> MAKQLQARRLDGIDYNPWVEFVKLASEHDVVNLGQGFPDFPPPDFAVEAFQHAVSGDFMLNQYTKTFGYPPLTKILASFFGELLGQEIDPLRNVLVTVGGYGALFTAFQALVDEGDEVIIIEPFFDCYEPMTMMAGGRPVFVSLKPGPIQNGELGSSSNWQLDPMELAGKFTSRTKALVLNTPNNPLGKVFSREELELVASLCQQHDVVCITDEVYQWMVYDGHQHISIASLPGMWERTLTIGSAGKTFSATGWKVGWVLGPDHIMKHLRTVHQNSVFHCPTQSQAAVAESFEREQLLFRQPSSYFVQFPQAMQRCRDHMIRSLQSVGLKPLIPQGSYFLITDISDFKRKMPDLPGAVDEPYDRRFVKWMIKNKGLVAIPVSIFYSVPH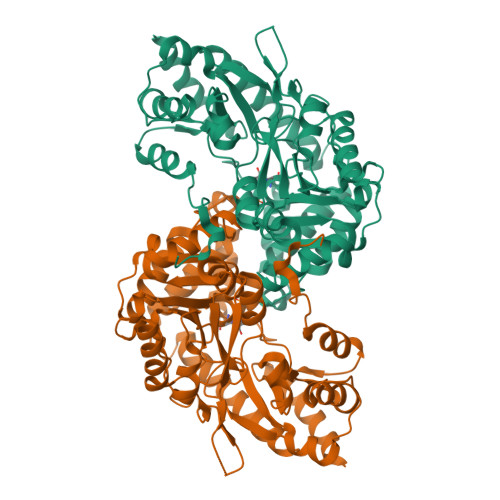QKHFDHYIRFCFVKDEATLQAMDEKLRKWKVEL>[2x]MIHHHHHHEHRHLKPFPPEFLWGAASAAYQVEGAWNEDGKGLSVWDVFAKQPGRTFKGTNGDVAVDHYHRYQEDVALMAEMGLKAYRFSVSWSRVFPDGNGAVNEKGLDFYDRLIEELRNHGIEPIVTLYHWDVPQALMDAYGAWESRRIIDDFDRYAVTLFQRFGDRVKYWVTLNEQNIFISFGYRLGLHPPGVKDM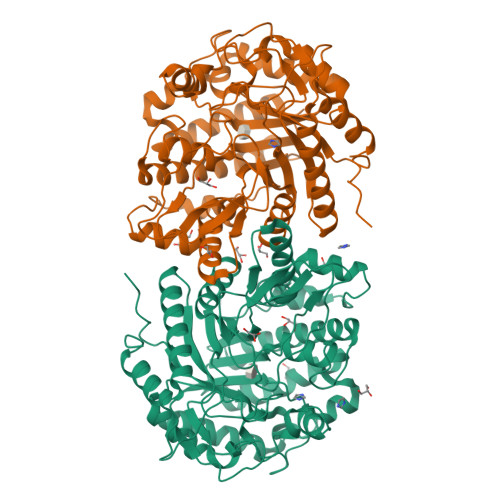KRMYEANHIANLANAKVIQSFRHYVPDGKIGPSFAYSPMYPYDSRPENVLAFENAEEFQNHWWMDVYAWGMYPQAAWNYLESQGLEPTVAPGDWELLQAAKPDFMGVNYYQTTTVEHNPPDGVGEGVMNTTGKKGTSTSSGIPGLFKTVRNPHVDTTNWDWAIDPVGLRIGLRRIANRYQLPILITENGLGEFDTLEPGDIVNDDYRIDYLRRHVQEIQRAITDGVDVLGYCAWSFTDLLSWLNGYQKRYGFVYVNRDDESEKDLRRIKKKSFYWYQRVIETNGAEL> YSKSPSNKDAALLEAARANNMQEVSRLLSEGADVNAKHRLGWTALMVAAINRNNSVVQVLLAAGADPNLGDDFSSVYKTAKEQGIHSLEVLITREDDFNNRLNNRASFKGCTALHYAVLADDYRTVKELLDGGANPLQRNEMGHTPLDYAREGEVMKLLRTSEAKYQEKQRKRELEHHHHHH

SKD3, also known as CLPB, is a ring-forming, ATP-fueled protein disaggregase essential for preserving mitochondrial integrity and structure. Ankyrin repeats are one of the most abundant motifs found in eukaryotic proteins and the Ank domain is the defining feature that distinguishes mammalian SKD3 from microbial Hsp100 unfoldases. Here, we present the atomic structures of the isolated Ank domains of SKD3 isoform-1 (ANKiso1) and SKD3 isoform-2 (ANKiso2). The two isoforms differ by a 30 amino acid stretch present in isoform-1 (exon-5), which represses the protein disaggregating activity of SKD3.

After solving the atomic structure of ANKiso1, we determined the 1.65-Å resolution crystal structure of ANKiso2. ANKiso2 crystallized as a monomer and is a monomer in solution. However, to our surprise, the structure of ANKiso2 markedly differs from the structure of ANKiso1 and is entirely α-helical with the long β-hairpin undergoing a conformational switch. Unlike ANKiso1, the crystal structure of ANKiso2 closely resembles the predicted AlphaFold2 model and superimposes with a root mean square deviation of only 0.541 Å over 143 Cα atoms. Notably, the concave surface that was previously occupied by the α5 helix is now bound by the C-terminal helix of a symmetry-related neighboring ANKiso2 domain. This interaction is totally fortuitous and could mimic an interaction with substrate that has displaced helix α5. Notably, this stretch is flanked by two β-strands that undergo conformational switching and form two α-helices in isoform-2, providing a structural basis for SKD3 activation by substrate. Although the basal ATPase activity of SKD3iso2 is reduced by half compared to isoform-1, we found that the ability of SKD3iso2 to recover functional protein from amorphous FFL aggregates is >4-fold higher than that of SKD3, and comparable to levels observed with the more powerful Hsp104 bi-chaperone system, indicating that helix α5 may indeed repress the protein disaggregating activity of isoform-1.> SNADEPILSFSPKTYSFRQDGRIKEVSVFTYHKKYNPDKHYIYVVRILREGQIEPSFVFRTFDEFQELHNKLSIIFPLWK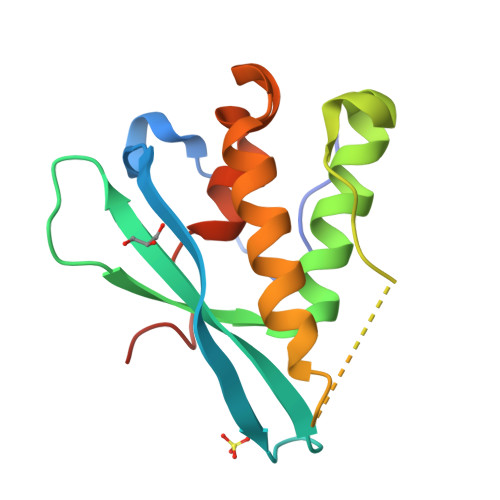LPGFPNRMVLGRTHIKDVAAKRKIELNSYLQSLMNASTDVAECDLVCTFFHPLLRDEKAEGIA> NMRVTQKLNHGWIFA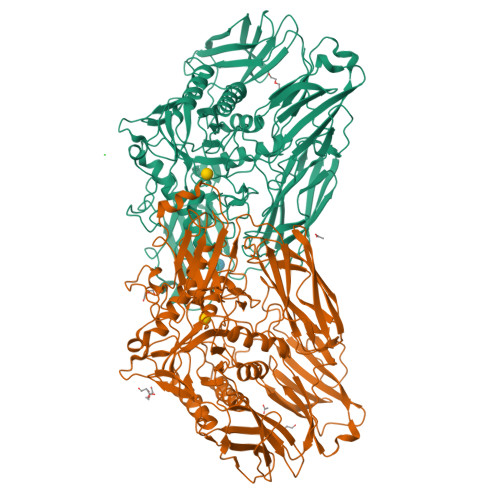EGAADPATPLAGETVTLPHNAVDLPLSYFDETSYQRAFTYQRVIAWDDAWQGRRVQLRFDGAMADNVVWVNGVQVVAHPDGYTPFVADLTDHLRPGDNLVTVRIDGSENPAIPPFGAQIDYLTYAGIYRDVWLMVLPERHLTNARILTPDALSDAKTVVIRPEVTAPGPVRARLLDGDREIAATEGEGELTLAGLTGLSLWSTDNPQLYTVELTLPDSGDVTTHRFGFRTAEWTPQGFLLNGQPMKLRGLNRHQSWAHQGYAAGRHAQERDAEIVRHDLCCNMVRTSHYPQSTWFLDRCDEIGLLVFEEIPGWQHIGDQAWQDRSVDNVRAMITRDWNHPSIVIWGVRINESPDNHDFYVRTNALARELDPTRAIGGVRCITDSEMLEDVYTMNDFILDESELPLINRPRTALRPTEEVTGIKKPVPYLVTEYNGHMFPTKAQDPELRQMEHVIRHLEVLNAAHGDPAISGCIGWCMFDYNTHKDFGAGDRICHHGVMDIWREPKFAAHAYGSQKPPSEGIVMEPVTFWARGERNIGGVLPLIVLTNCDEVEFECAGVTRRVGPDRERFPHLPRPPVIIDHRHISAEELGQWGMSWHPGRITGWLNGEQVALREYVADPLPTTLQIAPDRDTLPADGDIDLRVMLRALDQVGNRLPFLDAGIAVTVDGPARLIGPDLRMLQGGTTGMLLRLTGDAGTIRITARHPQFPEAVATVTVG;> MRVTQKLNHGWIFAEGAADPATPLAGETVTLPHNAVDLPLSYFDETSYQRAFTYQRVIAWDDAWQGRRVQLRFDGAMADNVVWVNGVQVVAHPDGYTPFVADLTDHLRPGDNLVTVRIDGSENPAIPPFGAQIDYLTYAGIYRDVWLMVLPERHLTNARILTPDALSDAKTVVIRPEVTAPGPVRARLLDGDREIAATEGEGELTLAGLTGLSLWSTDNPQLYTVELTLPDSGDVTTHRFGFRTAEWTPQGFLLNGQPMKLRGLNRHQSWAHQGYAAGRHAQERDAEIVRHDLCCNMVRTSHYPQSTWFLDRCDEIGLLVFEEIPGWQHIGDQAWQDRSVDNVRAMITRDWNHPSIVIWGVRINESPDNHDFYVRTNALARELDPTRAIGGVRCITDSEMLEDVYTMNDFILDESELPLINRPRTALRPTEEVTGIKKPVPYLVTEYNGHMFPTKAQDPELRQMEHVIRHLEVLNAAHGDPAISGCIGWCMFDYNTHKDFGAGDRICHHGVMDIWREPKFAAHAYGSQKPPSEGIVMEPVTFWARGERNIGGVLPLIVLTNCDEVEFECAGVTRRVGPDRERFPHLPRPPVIIDHRHISAEELGQWGMSWHPGRITGWLNGEQVALREYVADPLPTTLQIAPDRDTLPADGDIDLRVMLRALDQVGNRLPFLDAGIAVTVDGPARLIGPDLRMLQGGTTGMLLRLTGDAGTIRITARHPQFPEAVATVTVG> GPRP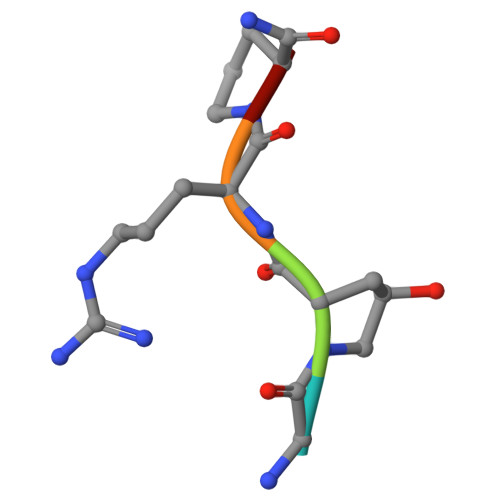X> GPHMASALVMKKGQRLSRDALRTQLDSAGYRHVDQVMEHGEYATRGALLDLFPMGSELP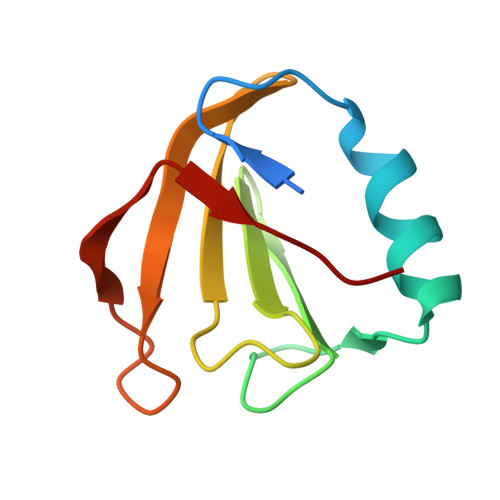YRLDFFDDEIDSLRVFDVDSQRTLEEVEAINLLP> MRGSHHHHHHGSIQKTTIAADSSSKPRGINYDTGIPFNVLIVDDSVFTVKQLTQIFTSEGFNIIDTAADGEEAVIKYKNHYPNIDIVTL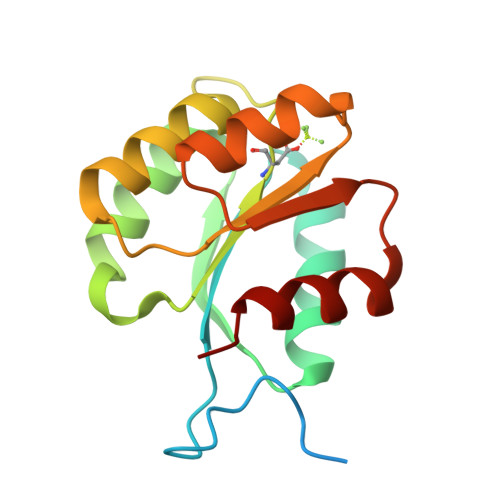DITMPKMDGITCLSNIMEFDKNARVIMISALGKEQLVKDCLIKGAKTFIVKPLDRAKVLQRVMSVFVK> KKGSFVEMVDNLRGKSGQGYYVEMTVGSPPQTLNILVDTGSSNFAVGAAPHPFLHRYYQRQLSSTYRDLRKGVYVPYTQGKWEGELGTDLVSIPHGPNVTVRANIAAITESDKFFINGSNWEGILGLAYAEI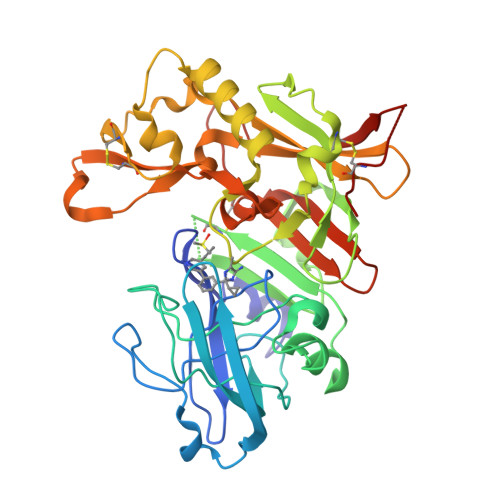ARPDDSLEPFFDSLVKQTHVPNLFSLQLCGGGSMIIGGIDHSLYTGSLWYTPIRREWYYEVIIVRVEINGQDLKMDCKEYNYDKSIVDSGTTNLRLPKKVFEAAVKSIKAASSTEKFPDGFWLGEQLVCWQAGTTPWNIFPVISLYLMGEVTNQSFRITILPQQYLRPVEDVATSQDDCYKFAISQSSTGTVMGAVIMEGFYVVFDRARKRIGFAVSACHVHDEFRTAAVEGPFVTLEDCGYN>[4x]MAKKTSSKGLKNPPGPWGWPLIGHM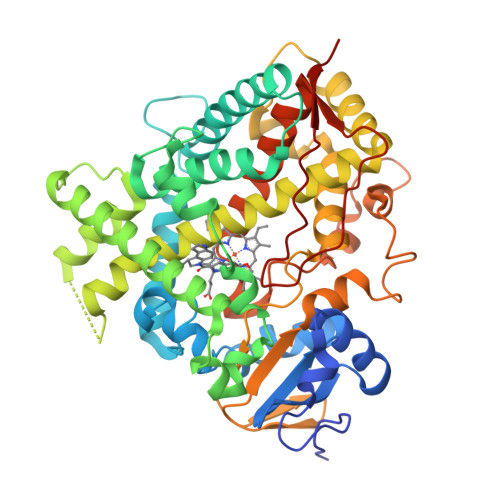LTLGKNPHLALSRMSQQYGDVLQIRIGSTPVVVLSGLDTIRQALVRQGDDFKGRPDLYTFTLISNGQSMSFSPDSGPVWAARRRLAQNGLKSFSIASDPASSTSCYLEEHVSKEAEVLISTLQELMAGPGHFNPYRYVVVSVTNVICAICFGRRYDHNHQELLSLVNLNNNFGEVVGSGNPADFIPILRYLPNPSLNAFKDLNEKFYSFMQKMVKEHYKTFEKGHIRDITDSLIEHCQEKQLDENANVQLSDEKIINIVLDLFGAGFDTVTTAISWSLMYLVMNPRVQRKIQEELDTVIGRSRRPRLSDRSHLPYMEAFILETFRHSSFVPFTIPHSTTRDTSLKGFYIPKGRCVFVNQWQINHDQKLWVNPSEFLPERFLTPDGAIDKVLSEKVIIFGMGKRKCIGETIARWEVFLFLAILLQRVEFSVPLGVKVDMTPIYGLTMKHACCEHFQMQLRSHHHHHH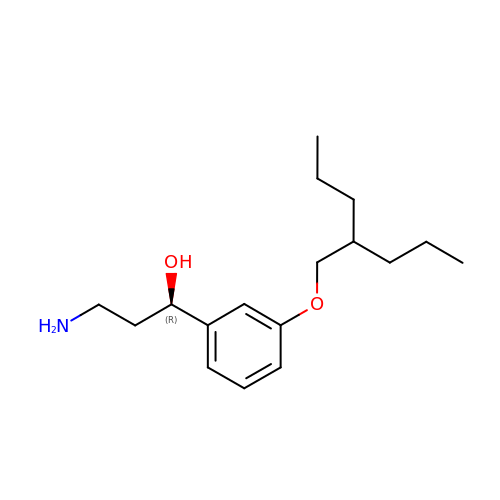(1R)-3-amino-1-{3-[(2-propylpentyl)oxy]phenyl}propan-1-ol | C17 H29 N O2 | LNRJYZXFMPBCCV-QGZVFWFLSA-N>TEEKTCDLVGEKGKESEKQLALLKRLTPLFQKSFESTVGQSPDMYSYVFRVCREAGQHSSGAGLVQIQKSNGKETVVGRFNETQIFQGSNWIMLIYKGGDEYDNHCGREQRRAVVMISCNRHTLAD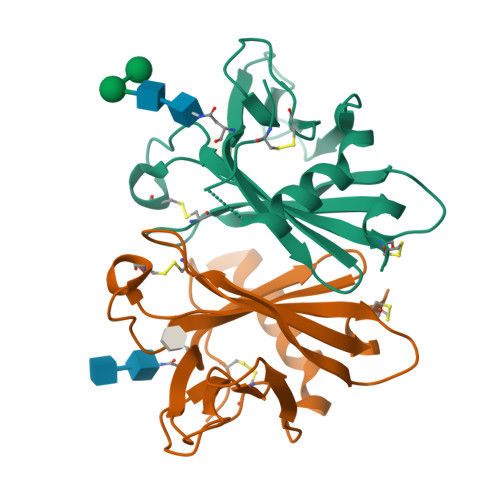NFNPVSEERGMVQDCFYLFEMDSSLACSHHHHHH[2x]>[4x]GSHMGVGSVAALLTVVFYIAAVMATNLYGATFPEWFGDLSKSLYTLFQVMTLESWSMGIVRPVMNVHPNAWVFFIPFIMLTTFTVLNLFIGIIVDAMAITKEQEEEAKTGHHQEPISQTLLHLGDRLDRIEKQLAQNNELLQRQQPQKK

Prokaryotic sodium channels are homotetramers, in which each monomer contains six transmembrane segments and is homologous to a single eukaryotic pseudorepeat. As with the eukaryotic channels, their S1–S4 segments form the voltage sensors, and the S5–S6 segments from each polypeptide chain associate to form an eight‐helix bundle that constitutes the pore. The selectivity filter (SF), which determines the channel's Na+ permeability over other cations, is formed by the close association of the P loops from each of the polypeptide chains.

The locations of three highly occupied sodium ion sites are seen in the centres of the selectivity filters, with ion B‐factors similar to those of the protein atoms. The crystallographic identification of these sites as arising from sodium ions is discussed in detail in the Appendix (including Appendix Figs S2, S3, S4, S5 and S6).> MMIRVAIGGPRGKMGQEAVHTVMNNENMELVAVLDHKDIGDLLSESPNFPASYEVPVFLNLESLIVTIKPDVFLDLTTPHQVFEHTMLCLQNNVRPVIGTTGFTDEQLQQCTILAEVNKLGCIVAPNFAIGAVLMMKFASLAAAYFPDVEIIEMHHDQKLDAPSGTAYKTAQMIAEVRPSHK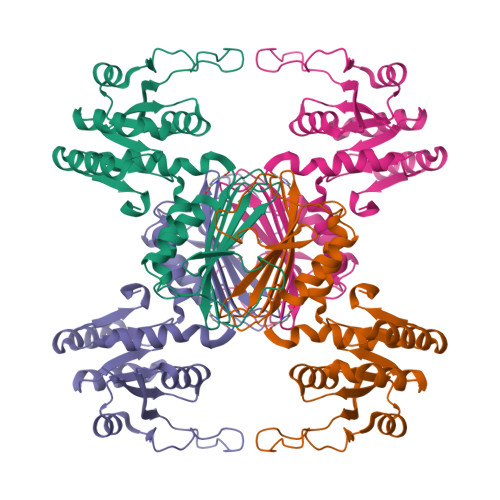QGHPNEKETLEGARGASYDGIPIHSVRLPGLIAHQQILFGGEGQLFTLRHDSYNRQSFMSGVTFSINQVMEIKELVYGLENIL1-(3-chlorophenyl)-3-(2-methoxyethyl)urea | C10 H13 Cl N2 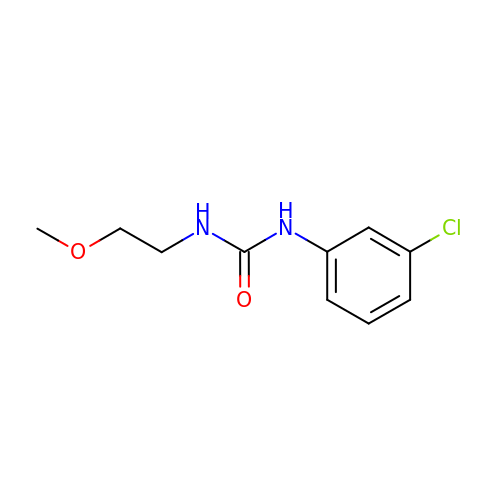O2 | OCWOGWHGSTYVMJ-UHFFFAOYSA-N> SNALLTSQIVDQYAEHIFYNSGAVGMALVVIDNNQVVNRSFGETQPGNNIRPRPDSLIRIASITKLMTSEIMVKLADDGIVKLTDPLKKYAPKGVNVPSYSAKQPIRLLHLASHTSGLPREQPGGPQKRPVFTWPTKDNRWQWLKLAKVTVPPGVKAAYSNLAY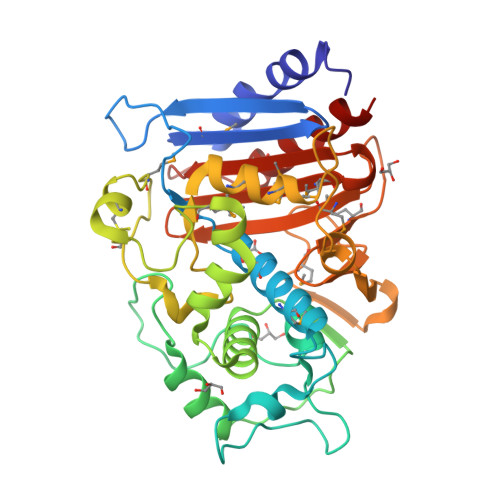DLLADALSRAAGKPYAHLLRDKITAPLGMKNTTLTPTAEQCKRLMIGVGSSRCGNTVAAAGSGGIYSTPEDMQHWMQQFLASDNSAPKRSAKREQALYFQRGDLVSLKGMDVAGQADALGLGWVYMAPKADLPGIMQKTGGGGGFITYMAMVPEKNIGVFVVVTRSQLTKFSNMSDGVNQLVAELVK> EQCVKKDELCIPYYLDCCEPLECKKVN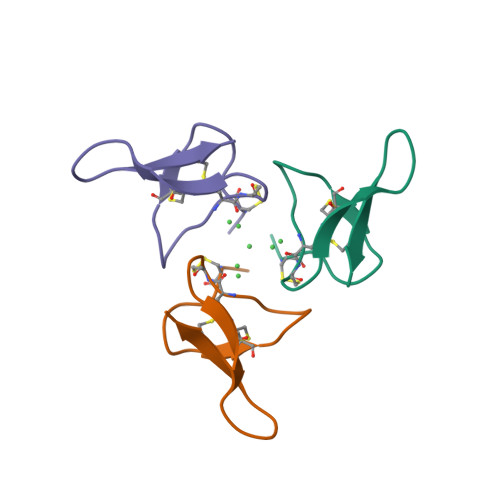WWDHKCIG> MHTAEFLETEPTEISSVLAGGYNHPLLRQWQSERQLTKNMLIFPLFISDNPDDFTEIDSLPNINRIGVNRLKDYLKPLVAKGLRSVILFGVPLIPGTKDPVGTAADDPAGPVIQGIK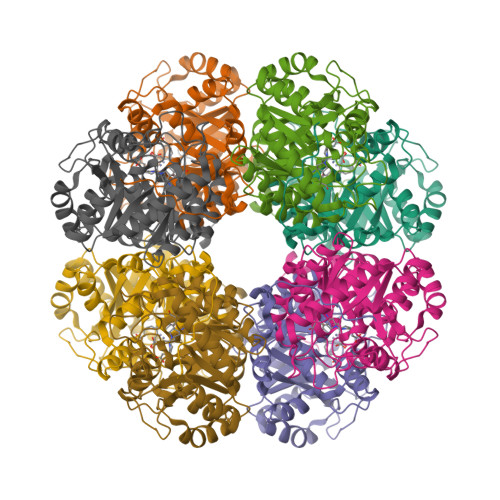FIREYFPELYIICDVCLCEYTSHGHCGVLYDDGTINRERSVSRLAAVAVNYAKAGAHCVAPSDMIDGRIRDIKRGLINANLAHKTFVLSYAAKFSGNLYGPFRDAACSAPSNGDRKCYQLPPAGRGLARRALERDMSEGADGIIVKPSTFYLDIMRDASEICKDLPICAYHVSGEYAMLHAAAEKGVVDLKTIAFESHQGFLRAGARLIITYLAPEFLDWLDE> NAKRDRIFVRVYNVMKRINCFINKNIKKSSTDSNYQLAVFMLMETMFFIRFG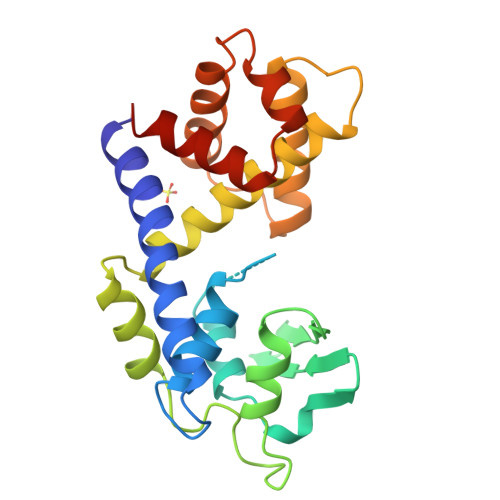KMKYLKENETVGLLTLKNKHIEISPDEIVIKFVGKDKVSHEFVVHKSNRLYKPLLKLTDDSSPEEFLFNKLSERKVYECIKQFGIRIKDLRTYGVNYTFLYNFWTNVKSISPLPSPKKLIALTIKQTAEVVGHTPSISKRAYMATTILEMVKDKNFLDVVSKTTFDEFLSIVVDHVKSSTDG N-{4-[(1E)-N-(N-hydroxycarbamimidoyl)ethanehydrazonoyl]phenyl}-7-nitro-1H-indole-2-carboxamide | C18 H17 N7 O4 | 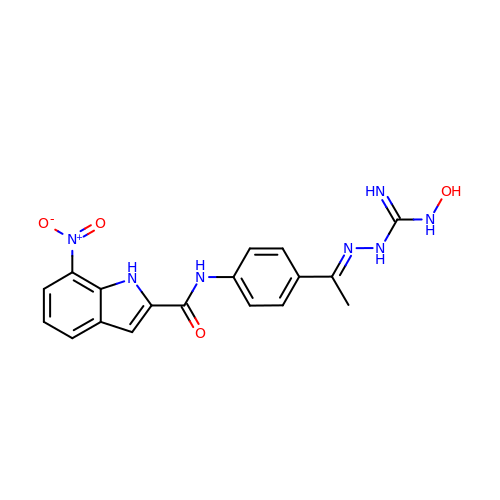CTGMEYONMRTKGL-LSHDLFTRSA-N>MAASGLDHLKNGYRRRFCRPSRARDINTEQGQNVLEILQDCFEEKSLANDFSTNSTKSVPNSTRKIKDTCIQSPSKECQKSHPKSVPVSSKKKEASLQFVVEPSEATNRSVQAHEVHQKILATDVSSKNTPDSKKISSRNINDHHSEADEEFYLSVGSPSVLLDAKTSVSQNVIPSSAQKRETYTFENSVNMLPSSTEVSVKTKKRLNFDDKVMLKKIEIDNKVSDEEDKTSEGQERKPSGSSQNRIRDSEYEIQRQAKKSFSTLFLETVKRKSESSPIVRHAATAPPHSCPPDDTKLIEDEFIIDESDQSFASRSWITIPRKAGSLKQRTISPAESTALLQGRKSREKHHNILPKTLANDKHSHKPHPVETSQPSDKTVLDTSYALIGETVNNYRSTKYEMYSKNAEKPSRSKRTIKQKQRRKFMAKPAEEQLDVGQSKDENIHTSHITQDEFQRNSDRNMEEHEEMGNDCVSKKQMPPVGSKKSSTRKDKEESKKKRFSSESKNKLVPEEVTSTVTKSRRISRRPSDWWVVKSEESPVYSNSSVRNELPMHHNSSRKSTKKTNQSSKNIRKKTIPLKRQKTATKGNQRVQKFLNAEGSGGIVGHDEISRCSLSEPLESDEADLAKKKNLDCSRSTRSSKNEDNIMTAQNVPLKPQTSGYTCNIPTESNLDSGEHKTSVLEESGPSRLNNNYLMSGKNDVDDEEVHGSSDDSKQSKVIPKNRIHHKLVLPSNTPNVRRTKRTRLKPLEYWRGERIDYQGRPSGGFVISGVLSPDTISSKRKAKENIGKVNKKSNKKRICLDNDERKTNLMVNLGIPLGDPLQPTRVKDPETREIILMDLVRPQDTYQFFVKHGELKVYKTLDTPFFSTGKLILGPQEEKGKQHVGQDILVFYVNFGDLLCTLHETPYILSTGDSFYVPSGNYYNIKNLRNEESVLLFTQIKR[2x];> MEEQPQMQDADEPADSGGEGRAGGPPQVAGAQAACSEDRMTLLLRLRAQTKQQLLEYKSMVDASEEKTPEQIMQEKQIEAKIEDLENEIEEVKVAFEIKKLALDRMRLSTALKKNLEKISRQSSVLMDNMKHLLELNKLIMKSQQESWDLEEKLLDIRKKRLQLKQASESKLLEIQTEKNKQKIDLDSMENSERIKIIRQNLQMEIKITTVIQHVFQNLILGSKVNWAEDPALKEIVLQLEKNVDMMHHHHHH;> MSPQKRVKNVQAQNRTSQGSSSFQTTLSAWKVKQDPSNSKNISKHGQNNPVGDYEHADDQAEEDALQMAVGYFEKGPIKASQNKDKTLEKHLKTVENVAWKNGLASEEIDILLNIALSGKFGNAVNTRILKCMIPATVISEDSVVKAVSWLCVGKCSGSTKVLFYRWLVAMFDFIDRKEQINLLYGFFFASLQDDALCPYVCHLLYLLTKKENVKPFRVRKLLDLQAKMGMQPHLQALLSLYKFFAPALISVSLPVRKKIYFKNSENLWKTALLAVKQRNRGPSPEPLKLMLGPANVRPLKRKWNSLSVIPVLNSSSYTKECGKKEMSLSDCLNRSGSFPLEQLQSFPQLLQNIHCLELPSQMGSVLNNSLLLHYINCVRDEPVLLRFYYWLSQTLQEECIWYKVNNYEHGKEFTNFLDTIIRAECFLQEGFYSCEAFLYKSLPLWDGLCCRSQFLQLVSWIPFSSFSEVKPLLFDHLAQLFFTSTIYFKCSVLQSLKELLQNWLLWLSMDIHMKPVTNSPLETTLGGSMNSVSKLIHYVGWLSTTAMRLESNNTFLLHFILDFYEKVCDIYINYNLPLVVLFPPGIFYSALLSLDTSILNQLCFIMHRYRKNLTAAKKNELVQKTKSEFNFSSKTYQEFNHYLTSMVGCLWTSKPFGKGIYIDPEILEKTGVAEYKNSLNVVHHPSFLSYAVSFLLQESPEERTVNVSSIRGKKWSWYLDYLFSQGLQGLKLFIRSSVHHSSIPRAEGINCNNQY;> MNQEDLDPDSTTDVGDVTNTEEELIRECEEMWKDMEECQNKLSLIGTETLTDSNAQLSLLIMQVKCLTAELSQWQKKTPETIPLTEDVLITLGKEEFQKLRQDLEMVLSTKESKNEKLKEDLEREQRWLDEQQQIMESLNVLHSELKNKVETFSESRIFNELKTKMLNIKEYKEKLLSTLGEFLEDHFPLPDRSVKKKKKNIQESSVNLITLHEMLEILINRLFDVPHDPYVKISDSFWPPYVELLLRNGIALRHPEDPTRIRLEAFHQ;> MDSYSAPESTPSASSRPEDYFIGATPLQKRLESVRKQSSFILTPPRRKIPQCSQLQEDVDPQKVAFLLHKQWTLYSLTPLYKFSYSNLKEYSRLLNAFIVAEKQKGLAVEVGEDFNIKVIFSTLLGMKGTQRDPEAFLVQIVSKSQLPSENREGKVLWTGWFCCVFGDSLLETVSEDFTCLPLFLANGAESNTAIIGTWFQKTFDCYFSPLAINAFNLSWMAAMWTACKMDHYVATTEFLWSVPCSPQSLDISFAIHPEDAKALWDSVHKTPGEVTQEEVDLFMDCLYSHFHRHFKIHLSATRLVRVSTSVASAHTDGKIKILCHKYLIGVLAYLTELAIFQIE;> MSVLRPLDKLPGLNTATILLVGTEDALLQQLADSMLKEDCASELKVHLAKSLPLPSSVNRPRIDLIVFVVNLHSKYSLQNTEESLRHVDASFFLGKVCFLATGAGRESHCSIHRHTVVKLAHTYQSPLLYCDLEVEGFRATMAQRLVRVLQICAGHVPGVSALNLLSLLRSSEGPSLEDL;> MDETVAEFIKRTILKIPMNELTTILKAWDFLSENQLQTVNFRQRKESVVQHLIHLCEEKRASISDAALLDIIYMQFHQHQKVWEVFQMSKGPGEDVDLFDMKQFKNSFKKILQRALKNVTVSFRETEENAVWIRIAWGTQYTKPNQYKPTYVVYYSQTPYAFTSSSMLRRNTPLLGQALTIASKHHQIVKMDLRSRYLDSLKAIVFKQYNQTFETHNSTTPLQERSLGLDINMDSRIIHENIVEKERVQRITQETFGDYPQPQLEFAQYKLETKFKSGLNGSILAEREEPLRCLIKFSSPHLLEALKSLAPAGIADAPLSPLLTCIPNKRMNYFKIRDKHHHHHH;>MEQANPLRPDGESKGGVLAHLERLETQVSRSRKQSEELQSVQAQEGALGTKIHKLRRLRDELRAVVRHRRASVKACIANVEPNQTVEINEQEALEEKLENVKAILQAYHFTGLSGKLTSRGVCVCISTAFEGNLLDSYFVDLVIQKPLRIHHHSVPVFIPLEEIAAKYLQTNIQHFLFSLCEYLNAYSGRKYQADRLQSDFAALLTGPLQRNPLCNLLSFTYKLDPGGQSFPFCARLLYKDLTATLPTDVTVTCQGVEVLSTSWEEQRASHETLFCTKPLHQVFASFTRKGEKLDMSLVS[2x];> MDAELAEVRALQAEIAALRRACEDPPAPWEEKSRVQKSFQAIHQFNLEGWKSSKDLKNQLGHLESELSFLSTLTGINIRNHSKQTEDLTSTEMTEKSIRKVLQRHRLSGNCHMVTFQLEFQILEIQNKERLSSAVTDLNIIMEPTECSELSEFVSRAEERKDLFMFFRSLHFFVEWFEYRKRTFKHLKEKYPDAVYLSEGPSSCSMGIRSASRPGFELVIVWRIQIDEDGKVFPKLDLLTKVPQRALELDKNRAIETAPLSFRTLVGLLGIEAALESLIKSLCAEENN;> MSGKANASKKNAQQLKRNPKRKKDNEEVVLSENKVRNTVKKNKNHLKDLSSEGQTKHTNLKHGKTAASKRKTWQPLSKSTRDHLQTMMESVIMTILSNSIKEKEEIQYHLNFLKKRLLQQCETLKVPPKKMEDLTNVSSLLNMERARDKANEEGLALLQEEIDKMVETTELMTGNIQSLKNKIQILASEVEEEEERVKQMHQINSSGVLSLPELSQKTLKAPTLQKEILALIPNQNALLKDLDILHNSSQMKSMSTFIEEAYKKLDASHHHHHH;> MPVKRSLKLDGLLEENSFDPSKITRKKSVITYSPTTGTCQMSLFASPTSSEEQKHRNGLSNEKRKKLNHPSLTESKESTTKDNDEFMMLLSKVEKLSEEIMEIMQNLSSIQALEGSRELENLIGISCASHFLKREMQKTKELMTKVNKQKLFEKSTGLPHKASRHLDSYEFLKAILN;> MEEEAETEEQQRFSYQQRLKAAVHYTVGCLCEEVALDKEMQFSKQTIAAISELTFRQCENFAKDLEMFARHAKRTTINTEDVKLLARRSNSLLKYITDKSEEIAQINLERKAQKKKKSEDGSKNSRQPAEAGVVESEN;> MADHNPDSDSTPRTLLRRVLDTADPRTPRRPRSARAGARRALLETASPRKLSGQTRTIARGRSHGARSVGRSAHIQASGHLEEQTPRTLLKNILLTAPESSILMPESVVKPVPAPQAVQPSRQESSCGSLELQLPEL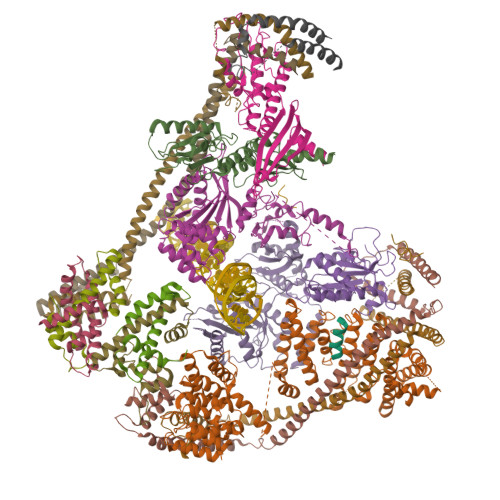EPPTTLAPGLLAPGRRKQRLRLSVFQQGVDQGLSLSQEPQGNADASSLTRSLNLTFATPLQPQSVQRPGLARRPPARRAVDVGAFLRDLRDTSLAPPNIVLEDTQPFSQPMVGSPNVYHSLPCTPHTGAEDAEQAAGRKTQSSGPGLQKNSPGKPAQFLAGEAEEVNAFALGFLSTSSGVSGEDEVEPLHDGVEEAEKKMEEEGVSVSEMEATGAQGPSRVEEAEGHTEVTEAEGSQGTAEADGPGASSGDEDASGRAASPESASSTPESLQARRHHQFLEPAPAPGAAVLSSEPAEPLLVRHPPRPRTTGPRPRQDPHKAGLSHYVKLFSFYAKMPMERKALEMVEKCLDKYFQHLCDDLEVFAAHAGRKTVKPEDLELLMRRQGLVTDQVSLHVLVERHLPLEYRQLLIPCAYSGNSVFPAQ;> MAPRGRRRPRPHRSEGARRSKNTLERTHSMKDKAGQKCKPIDVFDFPDNSDVSSIGRLGENEKDEETYETFDPPLHSTAIYADEEEFSKHCGLSLSSTPPGKEAKRSSDTSGNEASEIESVKISAKKPGRKLRPISDDSESIEESDTRRKVKSAEKISTQRHEVIRTTASSELSEKPAESVTSKKTGPLSAQPSVEKENLAIESQSKTQKKGKISHDKRKKSRSKAIGSDTSDIVHIWCPEGMKTSDIKELNIVLPEFEKTHLEHQQRIESKVCKAAIATFYVNVKEQFIKMLKESQMLTNLKRKNAKMISDIEKKRQRMIEVQDELLRLEPQLKQLQTKYDELKERKSSLRNAAYFLSNLKQLYQDYSDVQAQEPNVKETYDSSSLPALLFKARTLLGAESHLRNINHQLEKLLDQG;> MALSTIVSQRKQIKRKAPRGFLKRVFKRKKPQLRLEKSGDLLVHLNCLLFVHRLAEESRTNACASKCRVINKEHVLAAAKVILKKSRG;> MEGAGAGSGFRKELVSRLLHLHFKDDKTKVSGDALQLMVELLKVFVVEAAVRGVRQAQAEDALRVDVDQLEKVLPQLLLDF>MLEQMISSSKVGVKINEWYKYIRLFSVPDSEILKAEVEEEIRHMKEDHDLLLYYSLMCFRHQLMLDYLEPKTLNEERPKISDLLEKIESSQTDLKGILEYYFNFFRGMYEFEQYEYLNAISFYKQAERKLSLVADEIERAEFHYKVAEIYYHMKQTHMSMHHIVQAIDSYKAHENYTVRVIQCSFVIGLNYLDMDYPEKAIPHFKNALDKAREIDMSRLIGSSLYNLGLCSFAEEAYEKASEYFKEGIRVYQDNGYEHSNRILDILLMLTKTTFKMRNHSEGISWCAHGLSLSKNLNDEIMAKMFEFIHALYVDNDNEKLNSILNYLELKSMLSDVEDLASDAAKYYNEKEDHKVAVAYYEKVLYARKQIQRGDCLYET[2x];>RRGHTAS[2x]

Proteins of the RRNPPA family are the most frequent pheromone receptors in Bacillota and use small secreted oligopeptides as pheromones. While most members of the RRNPPA family act as transcriptional factors through DNA binding, Rap receptors are specialized members that exhibit the capability to develop their function by interaction with specific protein targets. Binding of the pheromone produced from the propeptide, which is named Phr in this RRNPPA subfamily, induces Rap receptor inhibition. Our results reveal that distinct maturation processes generate multiple mature pheromones, which bind to receptors with varying affinities but produce identical structural and biological responses.

In addition to the 2 putative pheromones RRGHTA and SRGHTS, we included in the analysis an extended (RRGHTAS) and a shorter (RGHTS) version of the internal and C-terminal putative pheromones, respectively, that could represent alternative forms of their maturation. Only a 20% reduction in the affinity (EC50 = 6,70 nM) was observed for the possible maturation variant of the internal Phr3T pheromone (RRGHTAS) with an extra amino acid. To molecularly assess the differences in affinity and stabilization for the alternative peptides analyzed we solved the structures for Rap3T in complex with RRGHTAS, SRGHTS, and RGHTS. Meanwhile complexes with RRGHTAS and RGHTS peptides exhibited P21 space group and a Rap dimer in the asymmetric unit. Remarkably, these structures exhibited nearly identical conformations as confirmed by the low differences in the superimposition of their Cα atoms for either individual monomers or the complete dimers (RMSD 0.36–0.50), dispelling the notion of peptides eliciting divergent conformational shifts. Notice that the molecular conformational are due to peptide binding and not induced by the crystallization conditions since crystals were obtained in 2 different space groups and cell dimensions. Interestingly, the structure of the complex with RRGHTAS peptide showed that the additional Ser residue lacks electron density that prevented its building, supporting the idea that this residue does not participate in the binding and that RRGHTA is the genuine mature peptide version.> SNAMKLYIYDHCPFCVKARMIFGLKNIPVELNVLQNDDEATPTRMIGQKMVPILQKDDSRYLPESMDIVHYVDNLDGKPLLTGKRNPAIEEWLRKVNGYVNQLLLPRFAKSAFDEFSTPAARQYFIRKKEASSGSFDNHLAHSAGLIKKIGDDLRLLDKLIVQPNAVNGELSEDDIHLFPLLRNLTLVAGIH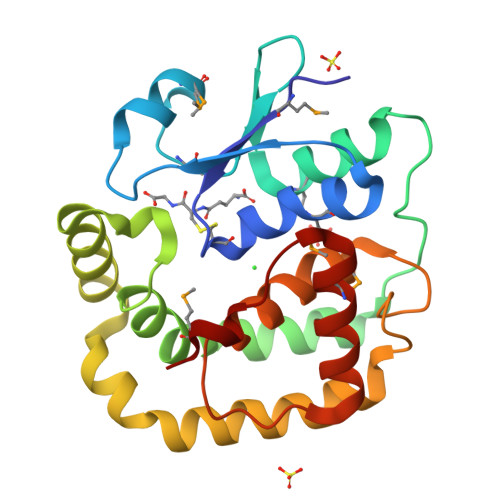WPTKVADYRDNMAKQTQINLLSSMAI> MASGTTTTAVKIGIIGGTGLDDPEILEGRTEKYVDTPFGKPSDALILGKIKNVDCVLLARHGRQHTIMPSKVNYQANIWALKEEGCTHVIVTTACGSLREEIQPGDIVIIDQFIDRTTMRPQSFYDGSHSCARGVCHIPMAEPFCPKTREVLIETAKKLGLRCHSKGTMVTIEGPRFSSRAESFMFRTWGADVINMTTVPEVVLAKEAGIC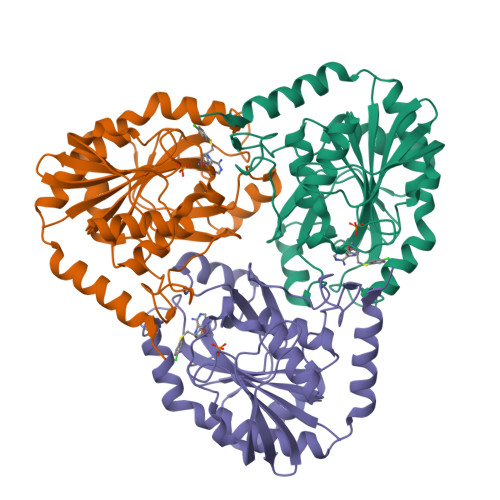YASIAMATDYDCWKEHEEAVSVDRVLKTLKENANKAKSLLLTTIPQIGSTEWSETLHNLKNMAQFSVLLPRH> MAEKVLVTGGAGYIGSHTVLELLEAGYLPVVIDNFHNAFRGGGSLPESLRRVQELTGRSVEFEEMDILDQGALQRLFKKYSFMAVIHFAGLKAVGESVQKPLDYYRVNLTGTIQLLEIMKAHGVKNLVFSSSATVYGNPQYLPLDEAHPTGGCTNPYGKSKFFIEEMIRDLCQADKTWNAVLLRYFNPTGAHASGCIGEDPQGIPNNLMPYVSQVAIGRREALNVFGNDYDTEDGTGVRDYI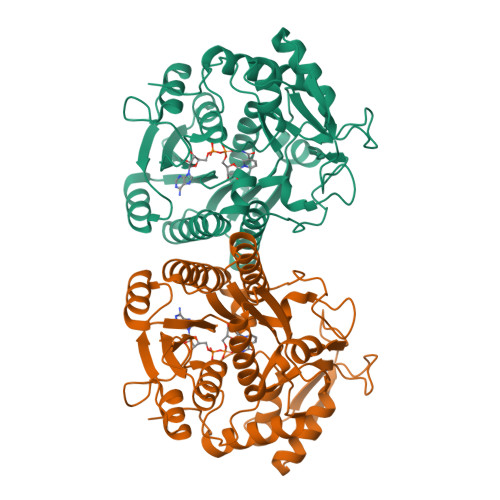HVVDLAKGHIAALRKLKEQCGCRIYNLGTGTGYSVLQMVQAMEKASGKKIPYKVVARREGDVAACYANPSLAQEELGWTAALGLDRMCEDLWRWQKQNPSGFGTQA> SNASADAQSFLNRVCGVSAARLTPCGTGTSTDVVYRAFDIYNDKVAGFAKFLKTNCCRFQEKDEDDNLIDSYFVVKRHTFSNYQHEETIYNLLKDCPAVAKHDFFKFRIDGDMVPHISRQRLTKYTMADLVYALRHFDEGNCDTLKEILVTYNCCDDDYFNKKDWYDFVENPDILRVYANLGERVRQALLKTVQFCDAMRNAGIVGVLTLDNQDLNGNWYDFGDFIQTTPGSGVPVVDSYYSLLMPILTLTRALTAESHVDTDLTKPYIKWDLLKYDFTEERLKLFDRYFKYWDQTYHPNCVNCLDDRCILHCANFNVLFSTVFPPTSFGPLVRKIFVDGVPFVVSTGYHFRELGVVHNQDVNLHSSRLSFKELLVYAADPAMHAASG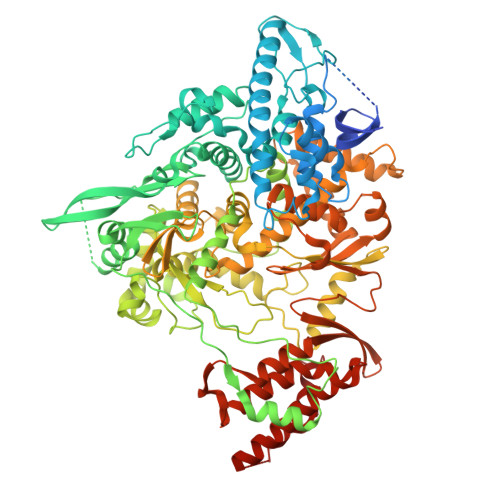NLLLDKRTTCFSVAALTNNVAFQTVKPGNFNKDFYDFAVSKGFFKEGSSVELKHFFFAQDGNAAISDYDYYRYNLPTMCDIRQLLFVVEVVDKYFDCYDGGCINANQVIVNNLDKSAGFPFNKWGKARLYYDSMSYEDQDALFAYTKRNVIPTITQMNLKYAISAKNRARTVAGVSICSTMTNRQFHQKLLKSIAATRGATVVIGTSKFYGGWHNMLKTVYSDVENPHLMGWDYPKCDRAMPNMLRIMASLVLARKHTTCCSLSHRFYRLANECAQVLSEMVMCGGSLYVKPGGTSSGDATTAYANSVFNICQAVTANVNALLSTDGNKIADKYVRNLQHRLYECLYRNRDVDTDFVNEFYAYLRKHFSMMILSDDAVVCFNSTYASQGLVASIKNFKSVLYYQNNVFMSEAKCWTETDLTKGPHEFCSQHTMLVKQGDDYVYLPYPDPSRILGAGCFVDDIVKTDGTLMIERFVSLAIDAYPLTKHPNQEYADVFHLYLQYIRKLHDELTGHMLDMYSVMLTNDNTSRYWEPEFYEAMYTPHTVLQ> GAMSANGKISVPEAVVNWLFKVIQPIYNDGRTTFHDSLALLDNFHSLRPRTRVFTHSDGTPQLLLSIYGTISTGE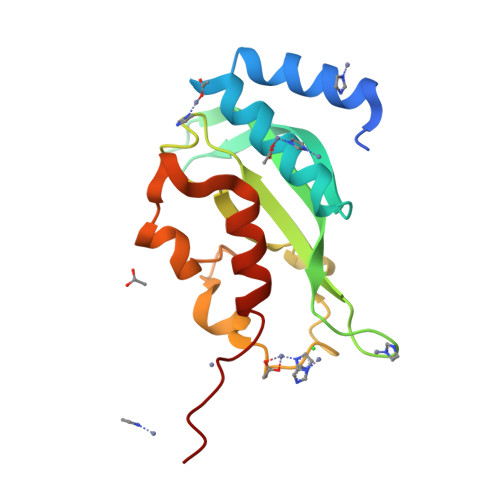DGSSPHSIPVIMWVPSMYPVKPPFISINLENFDMNTISSSLPIQEYIDSNGWIALPILHAWDPAAMNLIMVVQELMSLLHEPPQDQA>[2x]IIGGKKSDITKEPWAVGVLVDEKPFCGGSILTANFVITAAQC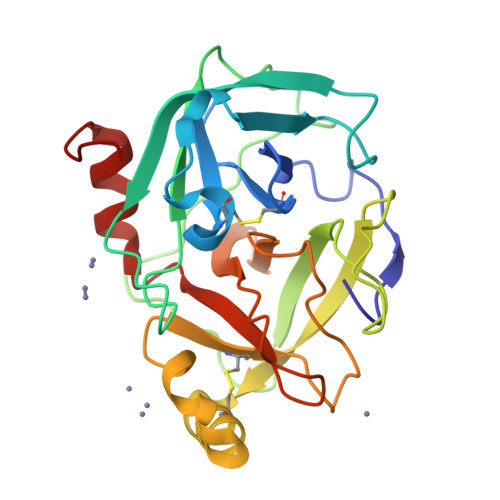VDGTKPSDISIHYGSSYRTTKGTSVMAKKIYIVRYHPLTMQNNYAVIETEMPIKLDDKTTKKIELPSLLYDPEPDTSVLVSGWGSTNFKSLEYSGDLMEANFTVVDRKSCEEQYKQIEADKYIYDGVFCAGGEYDETYIGYGDAGDPAVQNGTLVGVASYISSMPSEFPSVFLRVGYYVLDIKDIISGKVKPQ>SNAGPFIRPSYAQAGALKVGLLLPYSGTYAPLGEAITRGLELYVQSQGGKLGGRSISFVKVDDESAPPKATELTTKLIQSEKADVLIGTVHSGVAMAMVKIAREDGIPTIVPNAGADIITRAMCAPNVFRTSFANGQIGRATGDAMIKAGLKKAVTVTWKYAAGEEMVSGFKKSFTAGKGEVVKDITIAFPDVEFQSALAEIASLKPDCVYAFFSGGGALKFIKDYAAANLGIPLWGPGFLTDGVEAAAGPAGDGIKTVLHYVSDLDNAENQAFVKSFEAAYKIPPDVFAVQGWDAGQLLDAGVKAVGGDVAKRKELNAAMAAASFASPRGPFKLSAAHNPVQNFYLRELKGGKSVNLGLAA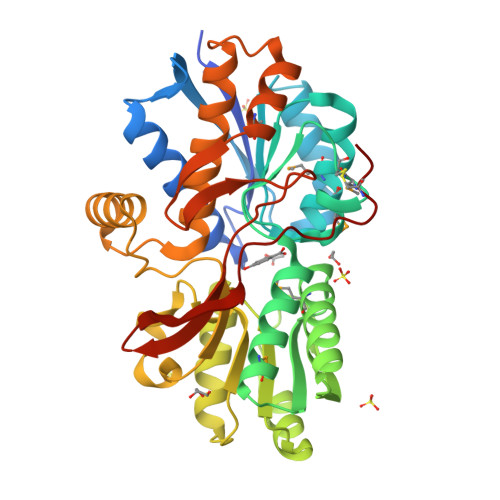PAVADEAIGCKLS[2x]>[6x]MHHHHHHHMAVLTQAKIGDSLAEFLVEATPDPKLRQLMMSMAEATRTIAHKVRTASCAGTACVNSFGDEQLAVDMVADKLLFEALKYSHVCKLACSEEVPEPVDMGGEGFCVAFDPLDGSSIVDTNFAVGTIFGVWPGDKLTNITGREQVAAGMGIYGPRTVF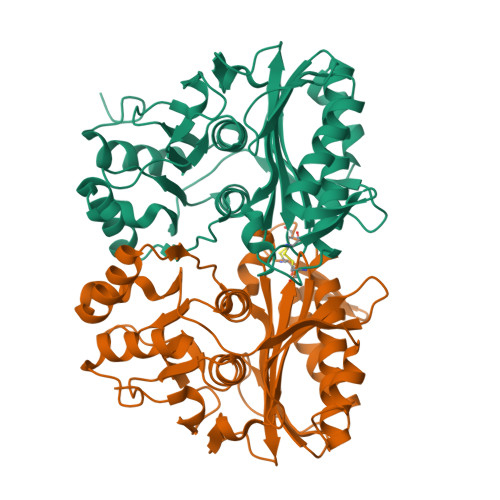CIALKDAPGCHEFLLMDDGKWMHVKETTHIGEGKMFAPGNLRATFDNPAYERLINFYLGEKYTLRYTGGMVPDVFQIIVKEKGVFTNVTSPTTKAKLRILFEVAPLALLIEKAGGASSCDGKAVSALDIPILVCDQRTQICYGSIGEVRRFEEYMYGTSPRFSEKVAA>MADFARSLSITTPEEMIEKAKGETAYLPCKFTLSPEDQGPLDIEWLISPADNQKVDQVIILYSGDKIYDDYYPDLKGRVHFTSNDLKSGDASINVTNLQLSD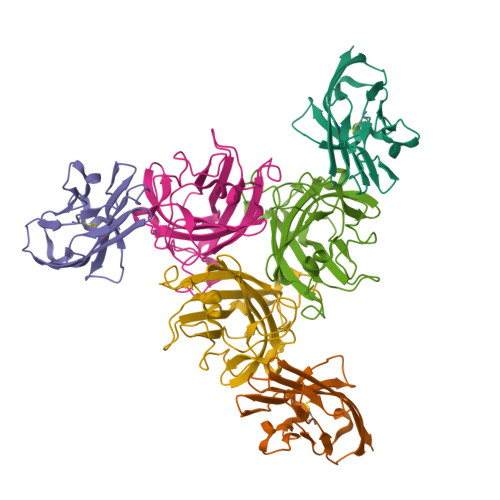IGTYQCKVKKAPGVANKKIHLVVLVK[12x];>[12x]MRGSHHHHHHGSPPAAPITLWTGPGPSINGFINDTPVIRCFICLTRDSNLVTVNASFVGEGGYRIVSPTQSQFSLIMEFDQFGQLMSTGNINSTTTWGEKPWGNNTVQPRPSHTWKLCMPNREVYSTPAATISRCGLDSIAVDGAPSRSIDCMLIINKPKGVATYTLTFRFLNFNRLSGGTLFKTDVLTFTYVGENQ The two gel-forming mucins MUC5AC and MUC5B constitute the main structural components of the mucus protecting the underlying epithelia in the respiratory system. The VWD assemblies are formed by the VWD domain, C8, trypsin inhibitor like (TIL) and E domains, except the VWD’ domain that only has the TIL and E domains. We determined the cryoEM structures of the wild type D3 assembly of the human MUC5AC mucin and the structural single nucleotide polymorphisms (SNP) variants Arg996Gln and Arg1201Trp that affect intermolecular interactions. The D3 assembly forms covalent dimers that can appear in two alternative conformations, open and closed, where the closed conformation dimers interact through an arginine-rich loop in the TIL3 domain to form tetramers.

The rs36189285 SNP corresponds to Arg996Gln, while rs878913005 corresponds to Arg1201Trp, both substituting the for MUC5AC typical arginines. The Arg996Gln mutation, located in VWD3 β9, is placed directly in the interface between the VWD3 and the TIL3 domain. The substitution results in a slight reduction of the distance between the two domains. No interactions involving this residue are observed in the WT or in Arg996Gln, but considering the resolution limitations a hydrogen bond between Arg996 or Gln996 and a TIL3 β1-β2 loop residue cannot be completely ruled out. Only when 2D templates from WT open conformation were used for particle picking, these could be detected in the Arg996Gln sample. The ratio in Arg996Gln dataset, 98:2, illustrates the important reduction in open conformation particles from 17% in the WT to only 2%. The open conformation was not detected in the D’D3CysD1 Arg99Gln cryoEM preparation during standard particle picking. Only template picking based on the WT open structure revealed a few particles. This observation, together with the described reduction of the distance between VWD3 and TIL3 domains, suggests that this mutation stabilizes the closed conformation and reduces the steric repulsion between Arg996 and TIL3. The mutation Arg996Gln, frequent in Asian population, affects the distance and the dynamics between the TIL3 domain and the VWD3, directly interfering in the conformational change and oligomerization.

>[2x]DAAQPARRAVRSSRHHHHHHGSPVCAAPMVFFDCRNATPGDTGAGCQKSCHTLDMTCYSPQCVPGCVCPDGLVADGEGGCITAEDCPCVHNEASYRAGQTIRVGCNTCTCDSRMWRCTDDPCLATCAVYGDGHYLTFDGQSYSFNGDCEYTLVQNHCGGKDSTQDSFRVVTENVPCGTTGTTCSKAIKIFLGGFELKLSHGKVEVIGTDESQEVPYTIQQMGIYLVVDTDIGLVLLWDKKTSIFINLSPEFKGRVCGLCGNFDDIAVNDFATRSRSVVGDVLEFGNSWKLSPSCPDALAPKDPCTANPFRKSWAQKQCSILHGPTFAACHAHVEPARYYEACVNDACACDSGGDCECFCTAVAAYAQACHEVGLCVSWRTPSICPLFCDYYNPEGQCEWHYQPCGVPCLRTCRNPRGDCLRDVRGLEGCYPKCPPEAPIFDEDKMQCVATCPTPPLPPRCHVHGKSYRPGAVVPSDKNCQSCLCTERGVECTYKAEACVCTYNGQRFHPGDVIYHTTDGTGGCISARCGANGTIERRVYPCSPTTPVPPTTFSFSTPPLVVSSTHTPSNGPSSAHTGPPSSAWPTTAGTSPRTRLPTASASLPPVCGEKCLWSPWMDVSRPGRGTDSGDFDTLENLRAHGYRVCESPRSVECRAEDAPGVPLRALGQRVQCSPDVGLTCRNREQASGLCYNYQIRVQCCTPLPCTSEQKLISEEDLSRKLTR>MEYFRYRGIIEGFYGKPWEHQERLDMFEFMQANNLNAYIYAPKQDLYHRELWREPYKEEQLQLFKELIEKAGSCGINFTFAISPGLSLVYSSEEELETLIRKITPFLEMGVHSIGIFFDNVPFDLIHEEDRNSYSNLAEAQADFLTRVLQRLESTISTPQIIMCPTFYCNDPNLEYLRILGQRLPKNIDVFWTGPNVCSHEITTSHMQEVQKSLQRPATLWDNYPVNDGGMMPELHIGPYDHRDPELHTHVVGIYANPMALPEASKLPLYTFAQYLNSPSQYNPQDSWRQAVSTLLGEDNLSAMEKFYQSNTISCLEPEEPAYLTNLFKKVQEDFASFRFEQGLRTLREEIISMQTTYSRLSTQDSKFFWEIRPWLEEYKLWTDYLDQAMITFSNLFTGFFTADEEQARESLQKALQGRTYLREVLKDAVDFRTRVCGDVVRNFLQQVLRSTVSIELQAEGKEWTALPPGI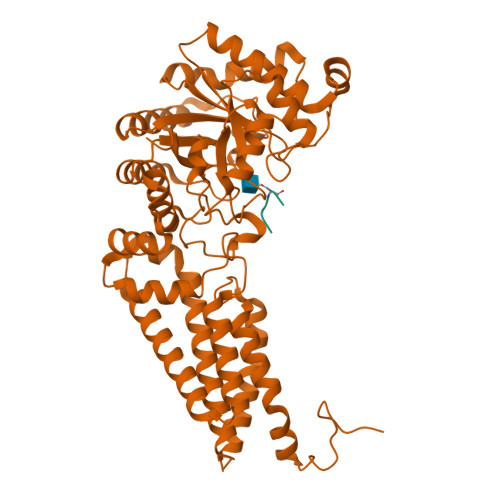VRD[2x];>VPYSSAQ[2x]>RGSHRILNLVKYDLYSIFKSPLTYLAILVVSSLIATQSILMANSMDNPKHIIVYGSVFAAAKWLLLIIGLMFVVKTITRDFSQGTIQLYMSKVKTRVGYIISKTISIILISILFALIHYVILIVVQASSNGKNLAFSKYVDNLWFFLIFLLFFGLFLFLITLASQKTAMIFSLGVFLVLIVPFIKPFITFIPRYGEKVLDAFDYIPFAYLTDKMISSNFDFSNWQWVISLGSIVIFFILNILYVAKKDI[2x];>MKLEHITKKYGSNVVLNDIDFDFGDSRIVGLIGKNGVGKTTVMKVMNGNIIKFDGKVDIDNADNIGFLIEHPKLYDNKSGLYNLKLFAQVLGKGFDKAYTDKIIDAFGMRPYIKKKVKKYSMGMKQKLAIAVSLMNKPKFLILDEPTNGMDPDGSIDVLTTIKSLVNELDM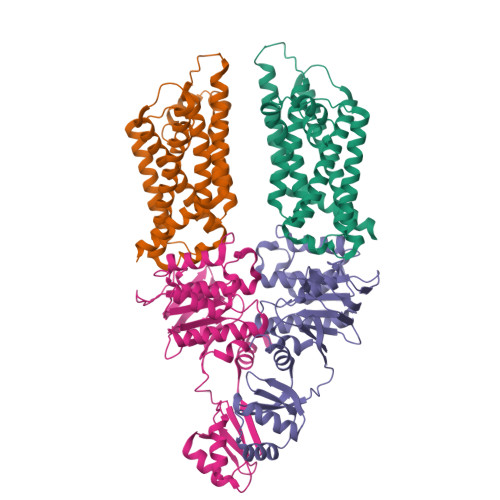RILISSHKLEDIELICDRAVFLRDGHFVQDVNMEEGVASDTTIVTVDHKDFDRTEKYLAEHFQLQNVDKADGHLMINAQKNYQVILKALSELDIYPKYIETRKSSLRDTYFNINQRGDK[2x]>GSSCEPGRTFDRCNTCRCGADGRSAACTLRACP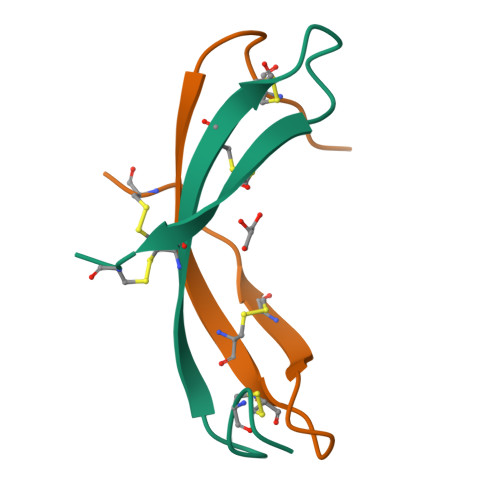NQ[4x]>MHHHHHHHHHHISSASGESQMSLDEIEDVYHTRPGYRPEEYRWGQGGAKIIDYHIQSAGVDFPPSLTGNQQTDFLMKVVFEYDFDCVVPGILIKTLDGLFLYGTNSFLASEGRENISVSRGDVRVFKFSLPVDLNSGDYLLSFGISAGNPQTDMTPLDRRYDSIILHVTKSMDFWGVID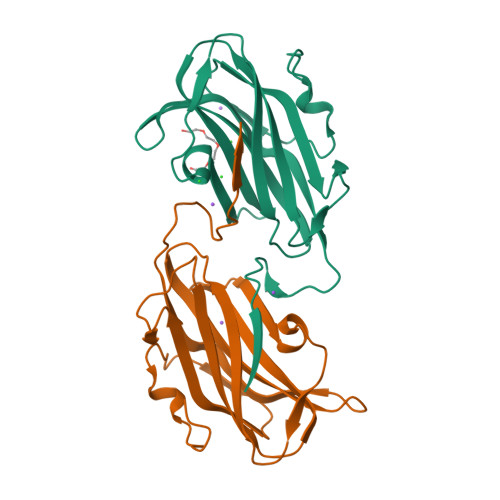LKSSFTSYQ[2x]>GPGMANTQKTLSLSVWTASSQERVRQDDPAGESLNIELFAARGEYESFQVALKAPEGEHRNVHFVVSDLKGTGDSFISKSNLTLYREHYVYISESSPQRGTVLPEGPGWYPDALIPFIDPATNEPPSGGELIAVPFALENNSNQVIWVDIQVPRDAEAGHYSGSYIVSSEHGEVTGQISLTVWNFELPLKPSLKSTFLIWSSRKKSTVEELLKHKLMCQQWNLSEEEKGAAPTSEGEWIEKYGVNCSGLGFWSKADTFNGVMPPPPTVEEIQAAASAHPSNLFLYNYTADEIGHYTSLYEPIKAWARNLHEAGVANLITMAPVPELYDDGSGSGRSAVDIWVILPLQYDKDRIQEVLAKGDEVWSYNCCVQDDYSPKWQIDFNPIEYRIQPGFINQSLGMTGILYWRVDFWTEDPWHDVLTLRADGMEFNGEGMLVYPGEQVGIDGVVPSIRLKAIRKGIEDYEYIEILKNLGHEQWALEISQSVGPDWHNWTKDHHKLEWARKQLGERINDLMTK[2x]

Beta-N-acetylgalactosaminidases (β-NGAs) hydrolyze the different β-GalNAc linkages of various glycans to modulate the length, combination, and abundance of glycans. Despite low sequence similarity, the crystal structures of these enzymes demonstrate that all enzymes share a prototype structure and have diversified their substrate specificities (oligosaccharide-releasing, oligosaccharide/monosaccharide-releasing, and monosaccharide-releasing) through the accumulation of mutations and insertional amino acid sequences. The overall structure of these enzymes is similar to that of CpNga123 and BvGH123, which consist of a β-sandwich domain at the N-terminus and a (β/α)8-barrel domain encompassing the catalytic region. Among Groups 1–4 and GH123, the DE motif is located at the same position, suggesting that these enzymes adopt the substrate-assisted catalysis reported for GH123 MR-β-NGAs.

Surprisingly, Group 1 NgaCa displayed strictly OR-type enzymatic activity and acted solely on Galβ1-3GalNAc-β-pNP. NgaCa in Group 1 had the simplest structure among the enzymes analyzed. The active site of NgaCa possesses a cleft shape that allows oligosaccharides to pass through to the −2 subsite, enabling oligosaccharide binding and OR-type β-NGA activity. Furthermore, three characteristic tryptophan residues (W197, W218, and W249) are located in the subsites −2 and −3. A docking model of NgaCa with oligosaccharide suggested that these tryptophan residues may play a role in a stacking-type interaction with sugars located in subsites −2 and −3. This structural feature indicated that Group 1 enzymes may act on the inner regions of longer sugar chains, in addition to disaccharides from the non-reducing end (e.g., Galβ1-3GalNAc-β-pNP). The increased number of residues could potentially reinforce substrate recognition in Group 4 and GH123 enzymes. Additional structural analyses (comparison of crystal structure with AlphaFold2 predicted structure of NgaCa, comparison of apo1-form and apo2-form of NgaCa, and comparison of GalNAc-thiazoline-bond form and GlcNAc-thiazoline-/apo-form of NgaAt, NgaDssm, and NgaP2) data are illustrated in Supplementary Fig. 13. The anomeric hydrogen signal of Galβ-1-3GalNAcβ-pNP (between the GalNAc and pNP moieties) disappeared within 1 min for NgaDssm and 10 min for NgaCa and Galβ-1-3GalNAcβ appeared, while Galβ-1-3GalNAcα anomeric signals appeared after 10 and 30 min, respectively, due to mutarotation. These results indicate that NgaDssm and NgaCa are anomer-retaining enzymes, similar to GH123 enzymes.>[2x]ANSVACRDGLRAQAECRNTTHLLQRQLTRTQDSLLQAETQANSCNLTVVTLQESLEKK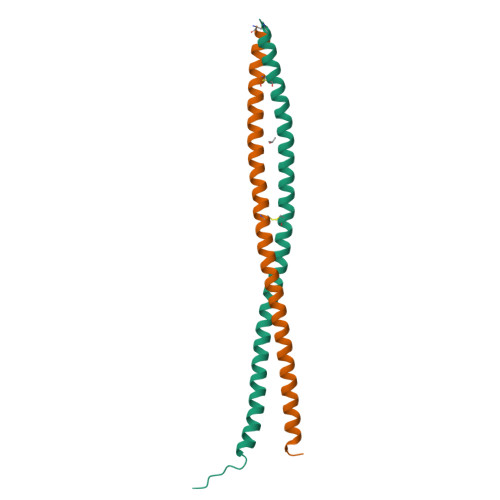VSQALEQQARIKELENEVTKLNQELENLRIQKETSSTVQVN>MAIRETVGVDGTPLVYSVTGDPDAR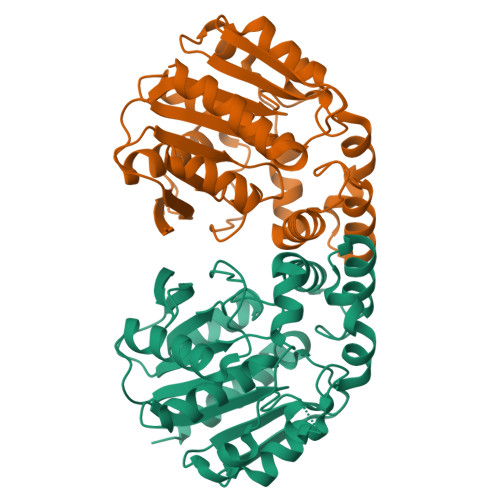ALVLLHGWAQSSKCWGPGVLDELAARYRVIAVDLRGHGYSGAPDTGYDDSAVWAGDVDAVLTAEGVTSGAVLLGWSYGGLVICDYLASNGTSAVDGVVLVGAITSIGRGEAGGKVGAAMRAAIPGAMSEEPREAIRALGAFGNALTGPPEGKGAQSQALFGASLTTPPRVRAALFNRSASHDDLLRSLDVPVLVLHGTEDSVVDVSAGRHAAELIPQARASFWEGCDHGPFVEDPERFVKEVGEFVDNLG[2x]>AHQDALPRLPVPPLQQSLDYYLKALQPIVSEEEWAHTKQLVDEFQTSGGVGERLQKGLERRAKKMENWLSEWWLKTAYLQFRQPVVIYSSPGVILPKQDFVDLQGQLRFAAKLIEGVLDFKSMIDNETLPVEFLGGQPLCMNQYY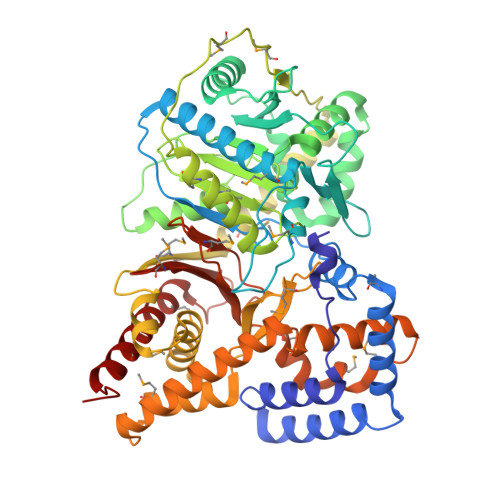QILSSCRVPGPKQDSVVNFLKSKRPPTHITVVHNYQFFELDVYHSDGTPLTSDQIFVQLEKIWNSSLQSNKEPVGILTSNHRNTWAKAYNNLIKDKVNRESVNSIQKSIFTVCLDKQVPRVSDDVYRNHVAGQMLHGGGSKFNSGNRWFDKTLQFIVAEDGSCGMVYEHAAAEGPPIVALVDHVMEYTKKPELVRSPMVPLPMPKKLRFNITPEIKNDIEKAKQNLSIMIQDLDIMMLTFHHFGKDFPKSEKLSPDAFIQVALQLAYYRIYGQACATYESASLRMFHLGRTDTIRSASIDSLAFVKGMGDSTVPEQQKVELLRKAVQAHRAYTDRAIRGEAFDRHLLGLKLQAIEDLVSMPDIFMDTSYAIAMHFNLSTSQVPAKTDCVMFFGPVVPDGYGICYNPMEAHINFSVSAYNSCAETNAARMAHYLEKALLDMRTLLQNHPRAK[2x]>[2x]GMVYVDPDRFDELVAEALDGIPEEFARAMRN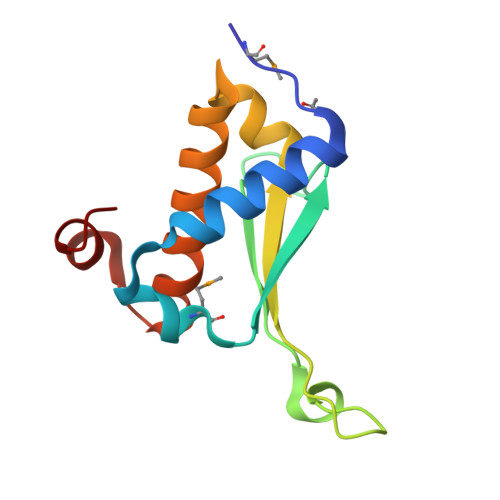VAVFVEDEPDDPELLGLYVGIPLTERTTAYGGVLPDRIIIYRNTICALCETESEVIDEVRKTVVHEIAHHFGIDDERLHELGY> MLPMITGFMNYGQQTLRAARYIGQGFMITLSHTNRLPVTIQYPYEKLITSERFRGRIHFEFDKCIACEVCVRVCPIDLPVVDWKLETNIRKKRLLNYSIDFGICIFCGNCVEYCPTNCLSMTE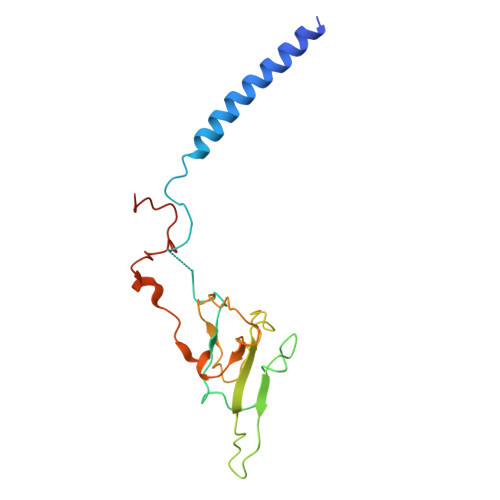EYEFSTYDRHELNYNQIALGRLPMSVIDDYTIRTIWNSPQTKNGVNPLI>GSHMALALVGEKIDRNRFTGEKIENSTFFNCDFSGADLSGTEFIGCQFYDRESQKGCNFSRAMLKDAIFKSCDLSMADFRNSSALGIEIRHCRAQGADFRGASFMNMITTRTWFCSAYITNTNLSYANFSKVVLEKCELWENRWIGAQVLGATFSGSDLSGGEFSTFDWRAANFTHCDLT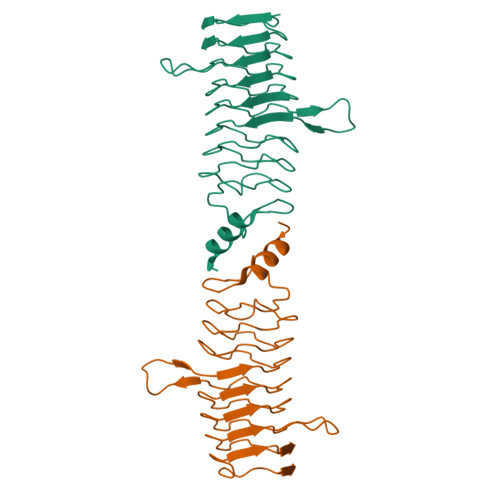NSELGDLDIRGVDLQGVKLDNYQASLLMERLGIAVIG[4x]>[4x]MKVGIDAGGTLIKIVQEQDNQRTFKTELTKNIDQVVEWLNQQQIEKLCLTGGNAGVIAENINIPAQIFVEFDAASQGLGILLKEQGHDLADYIFANVGTGTSLHYFDGQSQRRVGGIGTGGGMIQGLGYLLSQITDYKQLTDMAQHGDRNTIDLKVR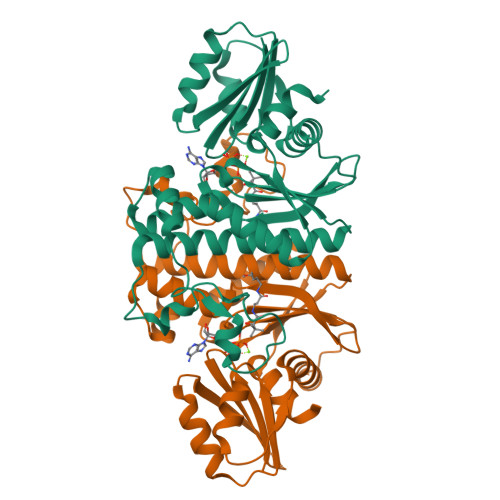HIYKDTEPPIPGDLTAANFGHVLHHLDADFTPSNKLAAVIGVVGEVVTTMAITVAREFKTENIVYIGSSFHNNALLRKVVEDYTVLRGCKPYYVENGAFSGAIGALYLE>MSSSVPTVKLFIGGKFVESKSDKWIDIHNPATNEVIGRVPQATKAEMDAAIASCKR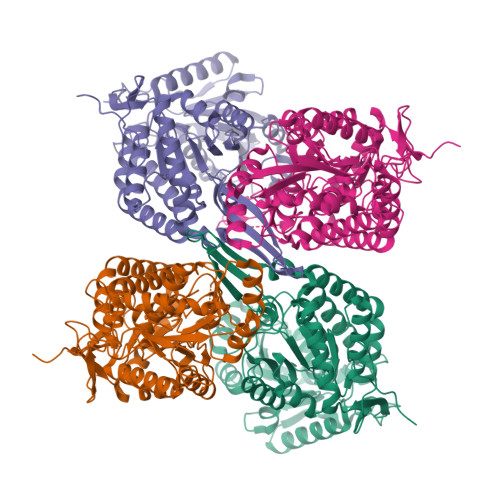AFPAWADTSVLSRQQVLLRYQQLIKENLKEIAKLITLEQGKTLADAEGDVFRGLQVVEHACSVTSLMMGETMPSITKDMDLYSHRLPLGVCAGIAPFNFPAMIPLWMFPMAMVCGNTFLMKPSERVPGATMLLAKLLQDSGAPDGTLNIIHGQHEAVNFICDHPDIKAISFVGSNKAGEYIFERGSRHGKRVQANMGAKNHGVVMPDANKENTLNQLVGAAFGAAGQRCMALSTAVLVGEAKKWLPELVEHAKNLRVNAGDQPGADLGPLITPQAKERVCNLIDSGTKEGASILLDGRKIKVKGYENGNFVGPTIISNVKPNMTCYKEEIFGPVLVVLETETLDEAIQIVNNNPYGNGTAIFTTNGATARKYAHLVDVGQVGVNVPIPVPLPMFSFTGSRSSFRGDTNFYGKQGIQFYTQLKTITSQWKEEDATLSSPAVVMPTMGRENLYFQ[4x]> MASTMPSYQGYILESAPVGATISESLNLTTPLRIVALDKDIEDTKDPELHLFLNDYTSVFTVTPTGITRYLTLLQPVDREEQQTYTFLITAFDGVQESEPVVVNIRVMDANDNTPTFPEISYDVYVYTDMSPGDSVIQLTAVDADEGSNGEISYEILVGGKGDFVINKTTGLVSIAPGVELIVGQTYALTVQASDNAPPAERRHSICTVYIEVLPPNNQSPPRFPQLMYSLEVSEAMRIGAILLNLQATDREGDPITYAIENGDPQRVFNLSETTGILSLGKALDRESTDRYILIVTASDGRPDGTSTATVNIVVTDVNDNAPVFDP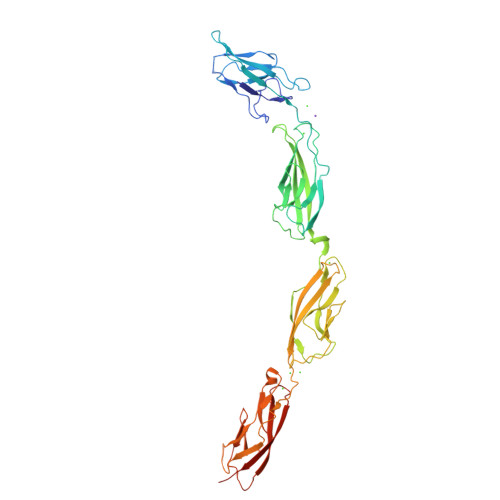YLPRNLSVVEEEANAFVGQVRATDPDAGINGQVHYSLGNFNNLFRITSNGSIYTAVKLNREARDHYELVVVATDGAVHPRHSTLTLYIKVLDIDLEHHHHHH> GMASMSVSTASTEMSVRKIAAHMKSNPNAKVIFMVGAGISTSCGIPDFRSPGTGLYHNLARLKLPYPEAVFDVDFFQSDPLPFYTLAKELYPGNFRPSKFHYLLKLFQDKDVLKRVYTQNIDTLERQAGVKDDLIIEAHGSFAHCHCIGCGKVYPPQVFKSKLAEHPIKDFVKCDVCGELVKPAIVFFGEDLPDSFSETWLNDSEWLREKITTSGKHPQQPLVIVVGTSLAVYPFASLPEEIPRKVKRVLCNLETVGDFKANKRPTDLIVHQYSDEFAEQLVEELGWQED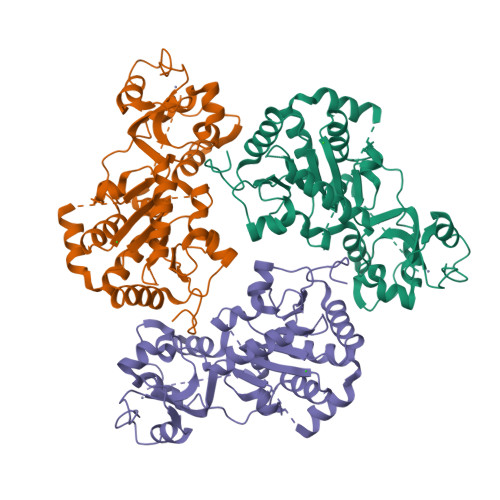FEKILTAQGGMGDNSKEQLLEIVHDLENLSLDQSEHESADKKDKKLQRLNGHDSDEDGASNSSSSQKAAKE> DVYQEPTDPKFPQQWYLSGVTQRDLNVKAAWAQGYTGHGIVVSILDDGIEKNHPDLAGNYDPGASFDVNDQDPDPQPRYTQMNDNRHGT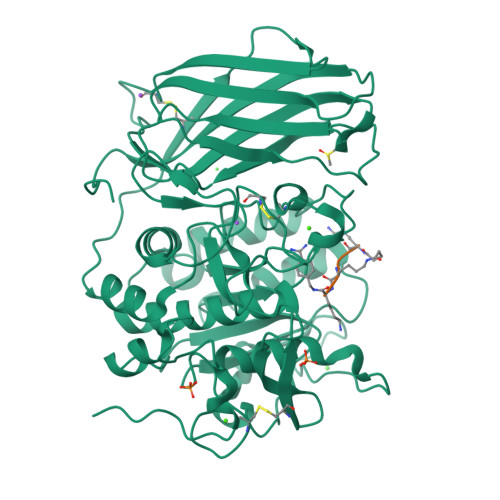RCAGEVAAVANNGVCGVGVAYNARIGGVRMLDGEVTDAVEARSLGLNPNHIHIYSASWGPEDDGKTVDGPARLAEEAFFRGVSQGRGGLGSIFVWASGNGGREHDSCNCDGYTNSIYTLSISSATQFGNVPWYSEACSSTLATTYSSGNQNEKQIVTTDLRQKCTESHTGTSASAPLAAGIIALTLEANKNLTWRDMQHLVVQTSKPAHLNANDWATNGVGRKVSHSYGYGLLDAGAMVALAQNWTTVAPQRKCIIDILTEPKDIGKRLEVRKTVTACLGEPNHITRLEHAQARLTLSYNRRGDLAIHLVSPMGTRSTLLAARPHDYSADGFNDWAFMTTHSWDEDPSGEWVLEIENTSEANNYGTLTKFTLVLYGTASGSLVPRGSHHHHHH;> RRKKX>[2x]GNEEETNNYTPVDNQSNSTSEIILQERNSSLPRVWSKKTAQRVTTRASFTDATDFLGCSYAVENGTSIIGDFANAKYPVVNMKKLLERYPSYINPKELRTTETKALSYSDFDRLEKNKTFTKTVKSGFSLNLGPFKFGRQKTIKETFVHNTDDSEKVVHGELSIEVVNGMLNLQTAPSALRKIAADYLDELFVDALYNSSMVELMQSYGEFVLTGYYTGGRASALFYGVDTNSIQFDSKEKDMDVAINASYEWKNKKPTAPSDTIHSASGNLSIGTKRENSETITNKFSALSYSIKTLGGAYGYSISTPPYDITNYSIDLTPWLQSLNDPKTHTMIDLQDGGLYPISDFILEENFKQRYNDTHMDFQYQESLEEPYIEIIKMYIRKSNSGEKLYDIVPVLNTRQGDKLIFSNPDAASQSDEELKANSIPATFLTKSNAIKDEKSKYYQLKIKADPNKTINPIIQTTLSFQINNVDEKGMYKFKNANTNIWYIYNPTSMYCFAYYDDDYIPDAYGILDWVNGIPIKAVTMTTLYQRYKIYGL

Membrane-attack complex/perforin (MACPF) proteins are transmembrane pore-forming proteins that are important in both human immunity and the virulence of pathogens. The crystal structure of a bacterial MACPF-domain-containing protein BT_3439 (Bth-MACPF) from B. thetaiotaomicron, a predominant member of the mammalian intestinal microbiota, has been determined. Bth-MACPF contains a membrane-attack complex/perforin (MACPF) domain and two novel C-terminal domains that resemble ribonuclease H and interleukin 8, respectively. The entire protein adopts a flat crescent shape, characteristic of other MACPF proteins, that may be important for oligomerization.

The data were indexed in the orthorhombic space group P212121 and the structure was determined at 2.46 Å resolution with two molecules per asymmetric unit using the MAD method. The final model of Bth-MACPF contains residues A/B36–558, 239 waters and other solvent molecules that were present in the crystallization or cryoprotection reagents, including one MPD [(4S)-2-methyl-2,4-pentanediol] molecule, one chloride ion and three ethylene glycol molecules. Furthermore, Bth-MACPF is likely to be a monomer in solution, as supported by crystal-packing analysis and analytical size-exclusion chromatography (data not shown). The MACPF domain contains two four-stranded β-sheets (A and B) in the central core, which is decorated by several helical insertions. Insertions between β1–β2 and β3–β4 (TMH1 and TMH2, respectively) correspond to the so-called TMH regions of CDCs, which unfold and form transmembrane β-hairpins. TMH1 (residues 126–173) contains one helix (αB) and two short 310-­helices that pack against the inner surface of the B sheet. TMH2 (residues 248–304) contains an antiparallel αβ–βα structure that sits on the outer surface of the B sheet. In contrast, D2 and D3 of Bth-MACPF, which are distant from the TMH regions, seem more likely to play a role in protein–protein interaction (e.g. polymerization or interaction with BT_3442) rather than membrane attachment. The shape of Bth-MACPF appears to be self-complementary, which could facilitate ring-like self-assembly to form pores across membranes. A model with 16 copies of Bth-MACPF forms a doughnut-shaped molecule with an inner radius of 110 Å, similar in pore size to the the C9 MACPF model.>[2x]ANVRLQHHHHHHHLEASDQRGYKPEDVAFDESFFSFGGHVGTSVEYEDKVTRGFNNTDKKEKTITNEVFNFFYNNPQWNFMGFYSFKIENREQKEPGYYENEDGIKQLFSLNKGHDLGNGWATGLIYELEYTRSKVYSPDVSGLRKNLAEHSIRPYLTYWNNDYNMGFYSNLEYLLSKEDRNAWGKRQEQGYSALFKPYKRFGNWEVGVEFYYQIKTNDEKQPDG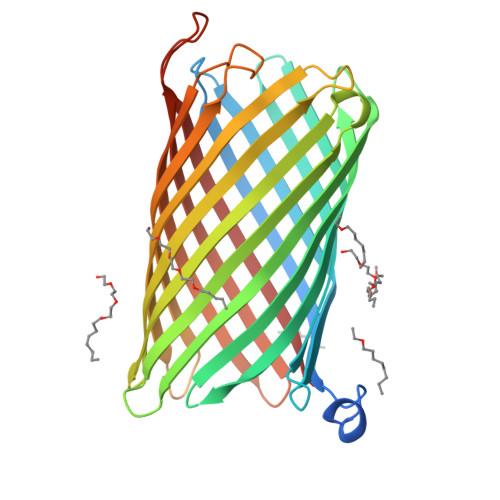TINEKSDFNERYIEPIVQYSFDDAGTLYTRVRVGKNETKNTDRSGGGNAGINYFKDIRKATVGYEQSIGESWVAKAEYEYANEVEKKSRLSGWEARNKSELTQHTFYAQALYRF>[2x]MAELLLVETPIPQQKHYESKPFPAVISPPSASIPIPALSLPLFTQTIKTQKHYLDSLLHESGAVLFRGFPVNSADDFNDVVEAFGFDELPYVGGAAPRTSVVGRVFTANESPPDQKIPFHHEMAQVREFPSKLFFYCEIEPKCGGET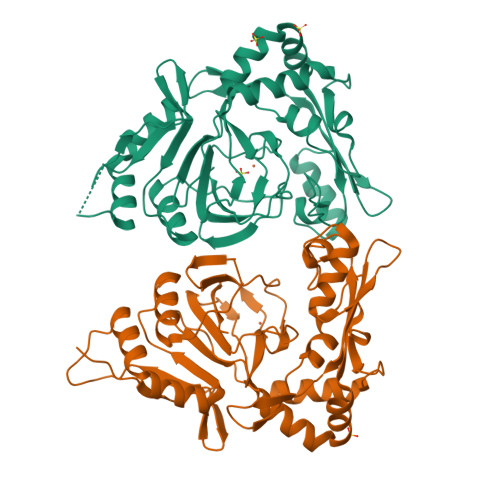PIVLSHVVYERMKDKHPEFVQRLEEHGLLYVRVLGEDDDPSSPIGRGWKSTFLTHDKNLAEQRAVDLGMKLEWTEDGGAKTVMGPIPAIKYDESRNRKVWFNSMVAAYTGWEDKRNDPRKAVTFGDGKPLPADIVHDCLRILEEECVAVPWQRGDVLLIDNWAVLHSRRPFDPPRRVLASLCK>[2x]DYLQQKRFLATSQGTTYVYDIPDMFRQMVERRWRECIEEGSVDGPQPDNVMTLVELVVEPDGERRVVEVTRLPGQNNVGMVAWRLTLYTPECPDGRDIVLIANDLTYYMGSFGPQEDWVYFKASQYARELKIPRIYISVNSGARIGVAEEVKSDFNVAWLDAERPERGFKYLYLTPEVYSKLGALGSVKTELIEDEGESRYRITDIIGKEDGLGVECLRDAGLIAGETAQAYEDIVTISIVTCRAIGIGSYIVRLGHRVIQVESSYIILTGYAALNKVLGRAVYASNNQLGGVQVMHHNGVSHAVAPSDLEAVRTALRWLAFVPKDKLSTVPILRVSDPVDRPVEWKPPRAAHDPRLMLAGDAARAGFFDVGSFDEIMQPWAQTVITGRARLGGIPVGVIAVETRTVELTQPADPANLDSEAKTLQQAGQVWFPDSAYKTAQAINDFSRENLPIMIFANWRGFSGGQKDMYEQILKFGAEIVRALRGATAPVLVYIPPGAELRGGAWAVVDPSVNSLRMEMYADPEARGGVLEAEGIVEVKFKQRDILKTMHRLDPELLRTGARISELKEQIKEISKGLDRRGSVDESLIRTDAGRAAETRVRELETELLAAEKTAKAREKELSPIYHEIAVQFAELHDTAERMLEKGCIFEIIPWRDSRRLFYWRLKRLLRQNEQERRVQAAVKPADNMQQGPAAATLRRWFTEDRGETQSHQWEHDNEAVCKWLEAQAGDDNSVLERNLRAIHQDALMQAVNNLVLELTPSQRSEFIRKLSALEMEQ

pmcAcetyl-coenzyme A carboxylases (ACCs) are crucial for fatty acid metabolism, facilitating the conversion of acetyl-CoA to malonyl-CoA, an essential step in fatty acid synthesis. In eukaryotes, ACCs are large, multidomain enzymes consisting of biotin carboxylase (BC), biotin carboxyl carrier protein (BCCP), and carboxyltransferase (CT) domains. The BC domain initiates the reaction by carboxylating the biotin group attached to BCCP, while the CT domain transfers the activated carboxyl group to acetyl-CoA, completing the conversion to malonyl-CoA. Mammals possess two ACC members: ACC1 in the cytosol of liver and adipose tissues and ACC2 associated with the mitochondrial outer membrane in the heart and muscle, whereas insects and other invertebrates have only one ACC gene.

Using cryo-EM on ACC isolated from a T. ni cell line, we obtained a 3.12 Å density map revealing the CT details. However, the 3.12 Å resolution cryo-EM density map revealed only the CT domain in high resolution and the CD domain in low resolution, with the other domains being invisible, likely due to the intrinsic dynamics and metastability of these domains in T. ni ACC. The solved ACC CT domain is full length, spanning from amino acid 1622 to 2396, with approximately 175 Å in diameter. CT forms a head-to-tail dimer, where the N domain of one monomer interacts with the C domain of the other. Both the N and C domains extensively interact with each other and with the ones from different protomers mainly by hydrophobic interactions and salt bridges. Additionally, when comparing the buried interface area among different species, single-cell organisms tend to have a lower buried interface, while human ACC CT exhibits the highest buried interface, with T. ni ACC CT nearly as extensive as the human ACC CT. The CT active site is located at the dimer interface (upper), necessitating dimerization for catalytic activity. We superimposed their structures onto our unbound CT structure and found that the interacting residues are largely conserved in T. ni ACC CT, with a few mutations that did not significantly change the pocket polarity. Our results show that the majority of the structure is largely conserved; however, the C terminus of the C domain (residues 2180–2230) in T. ni has elongated alpha helices. Additionally, we found that the CD domain of T. ni interacts with CT at a different angle, deviating approximately 45° counterclockwise from the angle in T. thermophila and around 30° clockwise from the angle in H. sapiens.> MDEKTKKAEEMALSLARAVAGGDEQAAI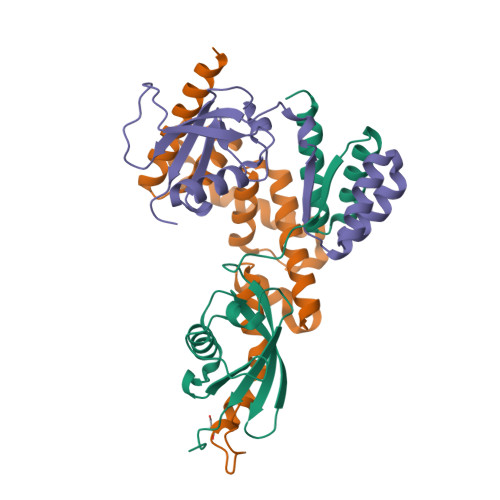KYATWLAEQRVPLRVQVKPEVSPTQDIRLCVSVEDAYMHTVTIWLTVRPDMTVASLKDMVFLDYGFPPSLQQWVVGQRLARDQETLHSHGIRRNGDGAYLYLLSARNTSLNP;> GRQDKMRKEGLQLVSMIQEGETAGASPEEVFSALQYSGTEVPLQWLRSELSYVLEMVAELAGQQDPELGAFSCQEARKAWLDRHGNLDEAVEECVRARRRKVHELQSLGFGPKEGSLQALFQHGGDVARALTELQRQRLEPFHQRLWDRDPEPTPCWD;> GPLGSPEFSSGNFKKEELATRLSQAIAGGDEKAAAQVAAVLAQHHVALNVQLMEAWFPPGPIRLQVTVEDATSVLSSSSSAHVSLKIHPHCSIAALQDQVFSEFGFPPAVQRWVIGRCLCMPERSLASYGVSQDGDPAFLYLLSAPREVSGQSLQNSKMDRKLGLFPQSLGLPHDLQPSSSSLPSPS> MHHHHHHKNIVNTSILSIVYKKDDLIDLSRYGAKINIGDRVYYDSIDKNQIKLINLESSTIEVILKNAIVYNSMYENFSTSFWIKIPKYFSKINLNNE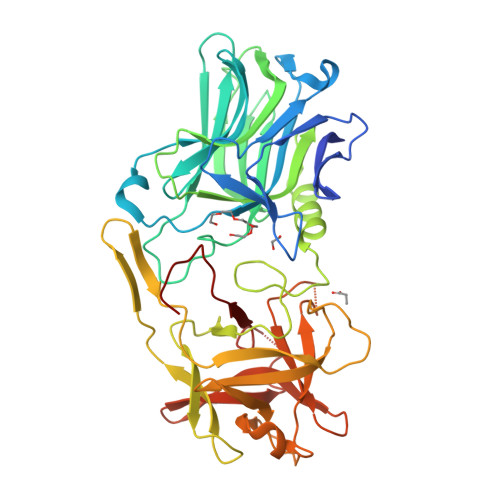YTIINCIENNSGWKVSLNYGEIIWTLQDNKQNIQRVVFKYSQMVNISDYINRWMFVTITNNRLTKSKIYINGRLIDQKPISNLGNIHASNKIMFKLDGCRDPRRYIMIKYFNLFDKELNEKEIKDLYDSQSNPGILKDFWGNYLQYDKPYYMLNLFDPNKYVDVNNIGIRGYMYLKGPRGSVMTTNIYLNSTLYMGTKFIIKKYASGNEDNIVRNNDRVYINVVVKNKEYRLATNASQAGVEKILSALEIPDVGNLSQVVVMKSKDDQGIRNKCKMNLQDNNGNDIGFVGFHLYDNIAKLVASNWYNRQVGKASRTFGCSWEFIPVDDGWGESSL>MKELIYIEEPSILFAHGQKCTDPRDGLALFGPLNQIYGIKSGVVGTQKGLQIFKSYLDKIQKPIYNHNNITRPMFPGFEAVFGCKWESQNIVFKEITDEEIRRYLFNASTHKRTY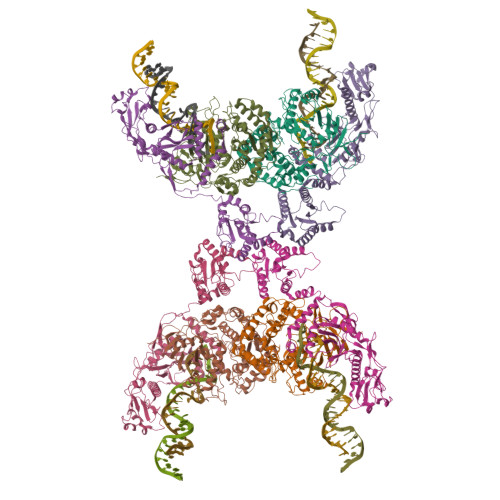DLVTLFNDKIITANKNDEERVDVWFVIVPEEIYKYCRPNSVLPNELVQTKSLISKSKAKSFRYTPTLFEEFNKKLKEVEKEAKTYNYDAQFHDQLKARLLEHTIPTQILRESTLAWRDFKNTFGAPIRDFSKIEGHLAWTISTAAYYKAGGKPWKLGDIRPGVCYLGLVYKKIEKSKNPQNACCAAQMFLDNGDGTVFKGEVGPWYNPEKGEYHLKPKEAKALLTQALESYKEQNKSYPKEVFIHARTRFNDEEWNAFNEVTPKNTNLVGVTITKSKPLKLYKTEGAFPIMRGNAYIVDEKKAFLWTLGFVPKLQSTLSMEVPNPIFIEINKGEAEIQQVLKDILALTKLNYNACIYADGEPVTLRFANKIGEILTASTEIKTPPLAFKYYI[4x];>MRNKIFISHATPEDDDFTRWLSLKLIGLGYEVWCDILFLDKGVDFWSTIEKEIRENTCKFLIVSSTAGNKREGVLKELAVATKVKKHLQDDMFIIPLAIDENLSYDDINIEIVRLNAIDFKKSWAKGLQDLLDAFEKQNVPKKPPDHSKSNLLYQQIFLHDKQAIEKEETYDSNWFPIISFPNELRFHRYDWRLPKQFDVRTLAFPAIRYKEYLCTFAWEYDFIHQLPKTETYNGQESIRISTSDILSGRYDTDFIRNYECQRLIVQLINKAFELRMKDKNVREYQMSKTFAYWIEKGKLEKDKFEKIKLVGKQKNKYWHFGISAAGKLYPSPVLMVSSHIIFTMDGINLIKSKSIQHSSRRKQGKNWWNDKWREKLLAFIRFLSDDQNAIYLNVGSEEKILISNKPLKFFGKMSYVTPSEVTLEEESVLADINNFEEDTEDLDELEDIE[4x]(4S,5S)-5-HYDROXY-2-METHYL-1,4,5,6-TETRAHYDROPYRIMIDINE-4-CARBOXYLIC ACID | C6 H10 N2 O3 | 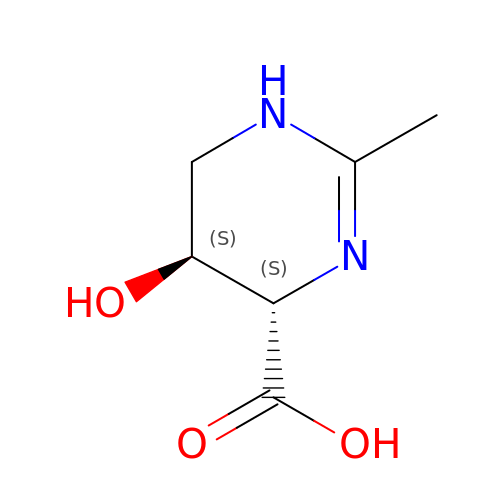KIIBBJKLKFTNQO-WHFBIAKZSA-N>[3x]MGQTVNEDSMDVKKENQEKTPQSSTSSVQRDDFHWEEYLKETGSISAPSECFRQSQIPPVNDFKVGMKLEARDPRNATSVCIATVIGITGARLRLRLDGSDNRNDFWRLVDSP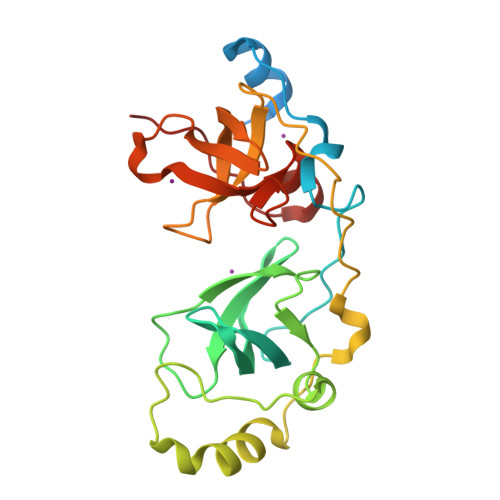DIQPVGTCEKEGDLLQPPLGYQMNTSSWPMFLLKTLNGSEMASATLFKKEPPKPPLNNFKVGMKLEAIDKKNPYLICPATIGDVKGDEVHITFDGWSGAFDYWCKYDSRDIFPAGWCRLTGDVLQPPGTS> DETKALKELYGPVDPTFLHRFYSLKAAVHGWKMVVCDKVRSLKLSDNNCYLNAVIMTLDLLKDIKFVIPALQHAFMKHKGGDSTDFIALIMAYGNCTFGAPDDASRLLHTVLAKAELCCSARMVWREWCNVCGIKDVVLQGLKACCYVGVQTVEDLRARMTYVCQCGGERHRQLVEHTTPWLLLSGTPNEKLVTTSTAPDFVAFNVFQGIETAVGHYVHARLKGGLILKFDSGTVSKTSDWKCKVTDVLFPGQKYSS

Pp1a and pp1ab are processed by two virus-encoded cysteine proteases, termed the papain-like protease (PLpro) and the 3C-like protease (3CLpro). Together, these two proteases cleave the polyproteins to produce 16 nonstructural proteins (nsps), which are essential for the formation of the replicase complex and hence RNA replication. SARS PLpro is a highly efficient deubiquitinating (DUB) enzyme having the ability to rapidly hydrolyze isopeptide bonds of proteins that are post-translationally modified by cellular ubiquitin-like (Ubl) molecules, such as ubiquitin (Ub) and interferon-stimulating gene 15 (ISG15), which are two key regulators of the innate immune response.

We also report the first X-ray crystal structure of a CoV PLpro or PLP2 without its flanking Ubl2 domain. The 60 amino acids encoding for the Ubl2 domain at the N-terminus and a single cysteine from the C-terminus of PLpro were removed. PLpro-ΔUbl2 crystallized in space group P 1 2 1 with one biologically active monomer in the asymmetric unit. X-ray data were collected to 1.95 Å, and the final X-ray data collection and refinement statistics are summarized in Table 1. The MERS-CoV PLpro-ΔUbl2 structure contains only the catalytic domain of PLpro with its three subdomains: thumb, fingers, and palm. Similar to the MERS PLpro-Ubl2 structure, the catalytic Cys111 in the MERS-CoV PLpro-ΔUbl2 structure is also modified by β-mercaptoethanol (BME) with a partial occupancy of 0.83. Due to the partially modified Cys111, His278 is observed to occupy at least one alternative position in order to accommodate the bulky, modified Cys111 residue. The MERS-CoV PLpro catalytic domain is observed to adopt a conformation that is nearly identical to the structure with the Ubl2 domain intact. The resulting root-mean-square-deviation (RMSD) is 0.4 Å when the Cα of 254 residues in PLpro-ΔUbl2 are aligned with Cα of 258 residues in PLpro-Ubl2. Truncation of the Ubl2 domain appears to cause only slight deviations in the ridge helix of the thumb domain due to the loss of two helix residues, Thr61 and Ala62.>[2x]HHHHHHMTTINPTNYTLLKKQ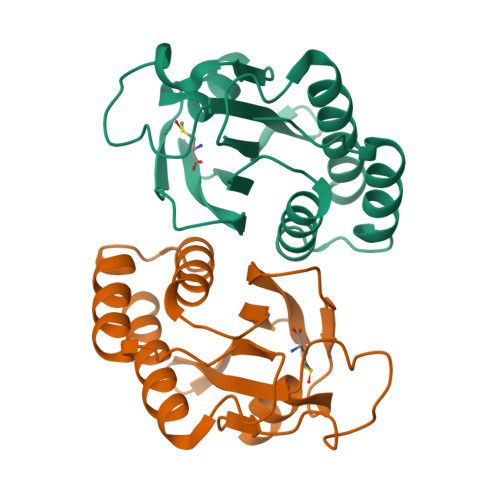AASLIEDEHHMIAILSNMSALLNDNLDQINWVGFYLLEQNELILGPFQGHPASVHIPIGKGVCGTAVSERRTQVVADVHQFKGHIACDANSKSEIVVPIFKDDKIIGVLDIDAPITDRFDDNDKEHLEAIVKIIEKQLA> GSGPIDFWSSHPGQSSAAERELIGRFQDRFPTLSVKLIDAGKDYDEVAQKFNAALIGTDVPDVVLLDDRWWFHFALSGVLTALDDLFGQVGVDTTDYVDSLLADYEFNGRHYAVPYARSTPLFYYNKAAWQQAGLPDRGPQSWSEFDEWGPELQRVVGAGRSAHGWANADLIS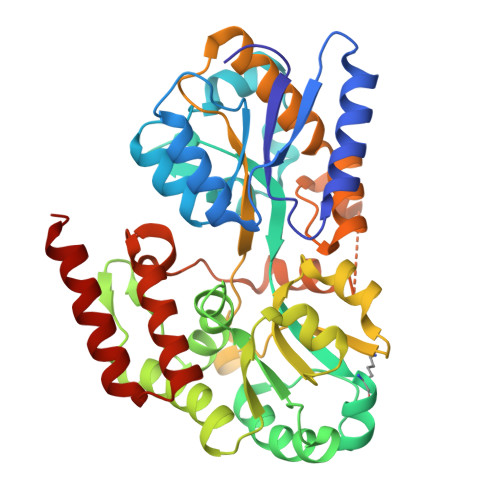WTFQGPNWAFGGAYSDKWTLTLTEPATIAAGNFYRNSIHGKGYAAVANDIANEFATGILASAVASTGSLAGITASARFDFGAAPLPTGPDAAPACPTGGAGLAIPAKLSEERKVNALKFIAFVTNPTNTAYFSQQTGYLPVRKSAVDRARVALDQLPHTRTQDYARVFLPGGDRIISAGLESIGLRGADVTKTFTNIQKRLQVILDRQI> YAEHKSHRGEYSVCDSESLWVTDKSSAIDIRGHQVTVLGEIKTGNSPVKQYFYETRCKEARPVKNGCRGIDDKHWNSQCKTSQTYVRALTSENNKLVGWR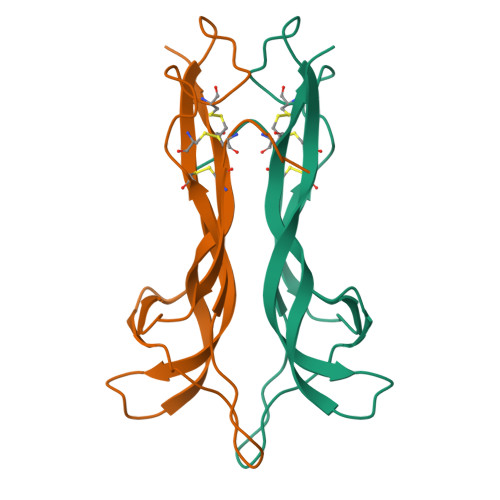WIRIDTSCVCALSRKIGRT> MGVPFFSSLRCMVDLGPCWAGGLTAEMKLLLALAGLLAILATPQPSEGAAPAVLGEVDTSLVLSSMEEAKQLVDKAYKERRESIKQRLRSGSASPMELLSYFKQPVAATRTAVRAADYLHVALDLLERKLRSLWRRPFNVTDVLTPAQLNVLSKSSGCAYQDVGVTCPEQDKYRTITGMCNNRRSPTLGASNRAFVRWLPAEYEDGFSLPYGWTPGVKRNGFPVALARAVSNEIVRFPTDQLTPDQERSLMFMQWGQLLDHDLDFTPEPAARASFVTGVNCETSCVQQPPCFPLKIPPNDPRIKNQADCIPFFRSCPACPGSNITIRNQINALTSFVDASMVYGSEEPLARNLRNMSNQLGLLAVNQRFQDNGRALLPFDNLHDDPCLLTNRSARIPCFLAGDTRSSEMPELTSMHTLLLREHNRLATELKSLNPRWDGERLYQEARKIVGAMVQIITYRDYLPLVLGPTAMRKYLPTYRSYNDSVDPRIANVFTNAFRYGHTLIQPFMFRLDNRYQPMEPNPRVPLSRVFFASWRVVLEGGIDPILRGLMATPAKLNRQNQIAVDEIRERLFEQVMRIGLDLPALNMQRSRDHGLPGYNAWRRFCGLPQPETVGQLGTVLRNLKLARKLMEQYGTPNNIDIWMGGVSEPLKRKGRVGPLLACIIGTQFRKLRDGDRFWWENEGVFSMQQRQALAQISLPRIICDNTGITTVSKNNIFMSNSYPRDFVNCSTLPALNLASWREAS;> GSTGSMKKTLVAGFAVAALS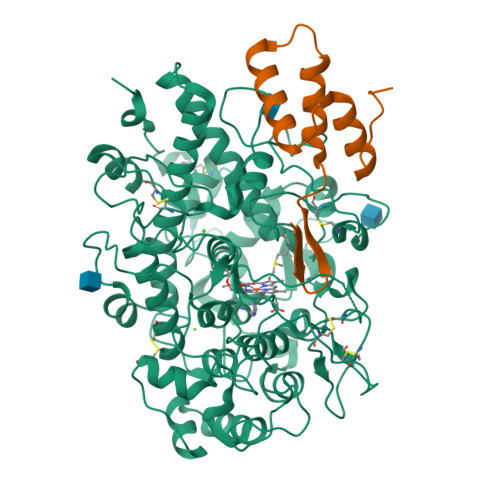TGIFAVSNEANAQVTSQNGIILHDDSRMLDHELQYVDVLINPNANPQTKERLKAYFESQGLNTVSEIVQKAKQDGLDTSKYDHLI> QAIKESYAFAVLGEPRYAFNFNHFDYVNPAAPKGGQITLSALGTFDNFNRYALRGNPGARTEQLYDTLFTTSDDEPGSYYPLIAESARYADDYSWVEVAINPRARFHDGSPITARDVEFTFQKFMTEGVPQFRLVYKGTTVKAIAPLTVRIELAKPGKEDMLSLFSLPVFPEKYWKDHKLSDPLATPPLASGPYRVTSWKMGQNIVYSRVKDYWAANLPVNRGRWNFDTIRYDYYLDDNVAFEAFKAGAFDLRMENDAKNWATRYTGKNFDKKYIIKDEQKNESAQDTRWLAFNIQRPVFSDRRVREAITLAFDFEWMNKALFYNAWSRTNSYFQNT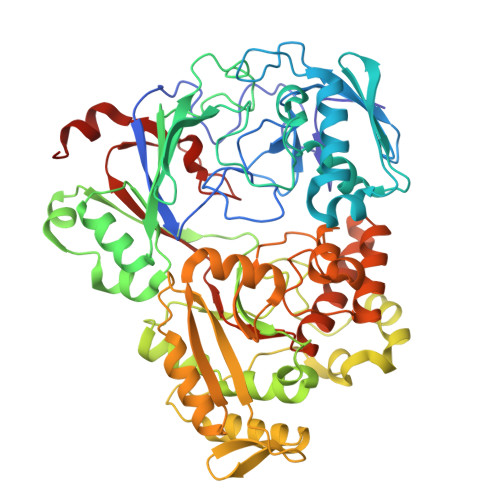EYAARNYPDAAELVLLAPMKKDLPSEVFTQIYQPPVSKGDGYDRDNLLKADKLLNEAGWVLKGQQRVNATTGQPLSFELLLPASSNSQWVLPFQHSLQRLGINMDIRKVDNSQITNRMRSRDYDMMPRVWRAMPWPSSDLQISWSSEYINSTYNAPGVQSPVIDSLINQIIAAQGNKEKLLPLGRALDRVLTWNYYMLPMWYMAEDRLAWWDKFSQPAVRPVYSLGIDTWWYDVNKAAKLPSASKQGE4'-{[(1R)-6-{2-[2-({N~5~-[N,N'-bis(tert-butoxycarbonyl)carbamimidoyl]-N~2~-(tert-butoxycarbonyl)-L-ornithyl}amino)ethoxy]ethoxy}-1-methyl-1-{2-oxo-2-[(1,3-thiazol-2-yl)amino]ethyl}-1,2,3,4-tetrahydroisoquinolin-7-yl]oxy}-2'-fluoro[1,1'-biphenyl]-4-carboxylic acid | C53 H69 F N8 O13 S | 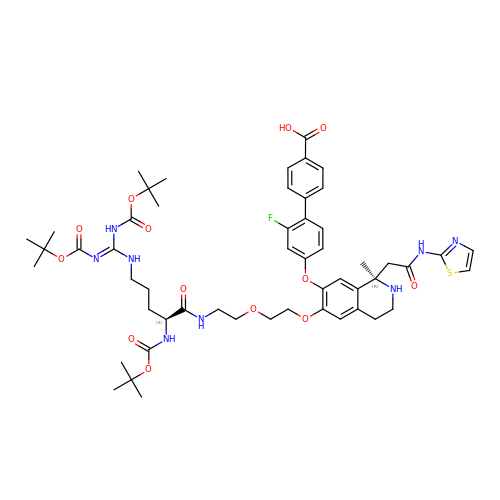BOAJXEFAPWTSFX-FXASYPJLSA-N>VVREAGEVVAIVPAAGSGERLAVGVPKAFYQLDGQTLIERAVDGLLDSGVVDTVVVAVPADRTDEARQILGHRAMIVAGGSNRTDTVN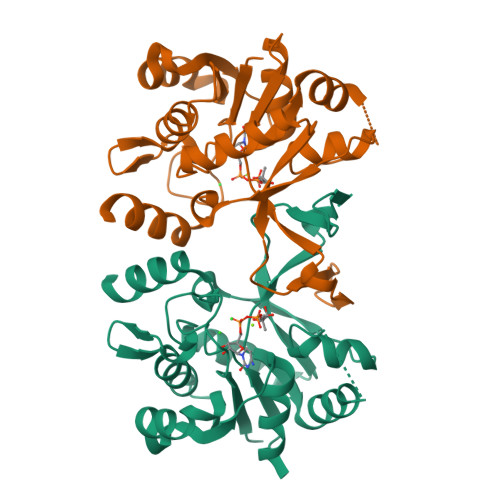LALTVLSGTAEPEFVLVHDAARALTPPALVARVVEALRDGYAAVVPVLPLSDTIKAVDANGVVLGTPERAGLRAVQTPQGFTTDLLLRSYQRGSLDLPAAEYTDDASLVEHIGGQVQVVDGDPLAFKITTKLDLLLAQAIVRG[2x]>HHHHFNLPPGNYKKPKLLYCSNGGHFLRILPDGTVDGTRDRSDQHIQLQLSAESVGEVYIKSTETGQYLAMDTDGLLYGSQTPNAECLFLERLEENHYNTYISKAHAEKNWFVGLKKNGSCKRGPRTH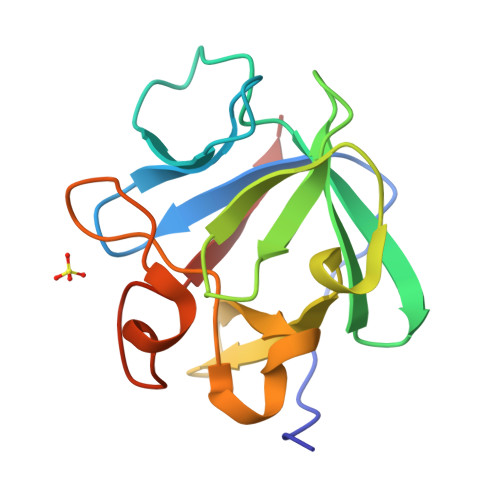YGQKAILFLPLPVSSD[2x]> MNLDTLLPLQTIREHAKCDDNPRVTDDLLKLYREAAFEAAELYTGLSFTPEKTIVEPIRLKGRRGKIILSATPIAGRPVVFYGGGLGSPLELIPRPGSNVLFFPYGSPDRFQTWGDCHTCDVESQLMATYVTGRRCENSVPAGIIIGILKLIAWNINNPGDEVMSVRNTLNANAQGLIGGTNN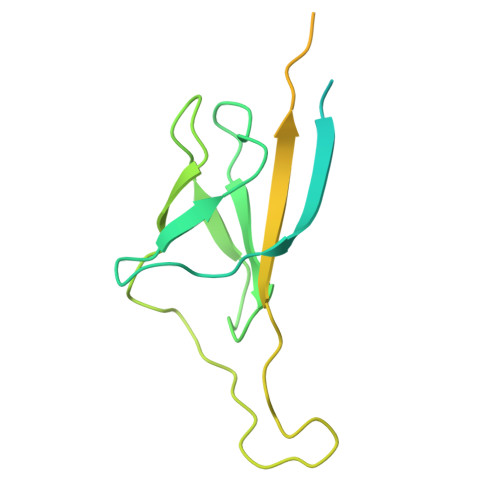GAVISGAQDEWFRYRRVLL> MGSSHHHHHHSQDPNSSSARLQVEMGDKFGEGRDPYLYPGLDIMRNRLNIHQQQRLEQAAYEMTALRAATIELGPLVRRLPHLRTIHRQLYQDIFDWAG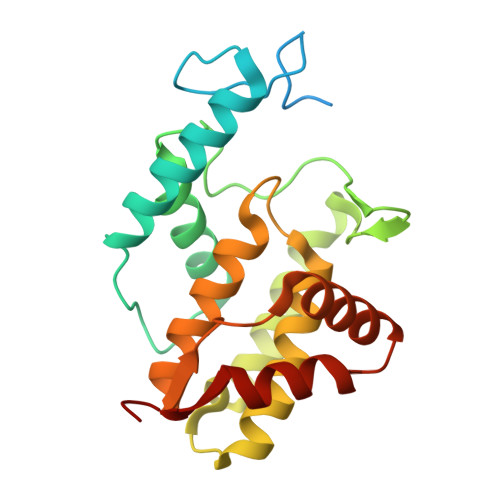QLREVDIYQGDTPFCHFAYIEKEGNALMQDLEEEGYLVGLEKAKFVERLAHYYCEINVLHPFRVGSGLAQRIFFEQLAIHAGYQLSWQGIEKEAWNQANQSGAMGDLTALQMIFSKVVSEAGESE5-hydroxypentyl alpha-D-glucopyranoside | C11 H22 O7 | 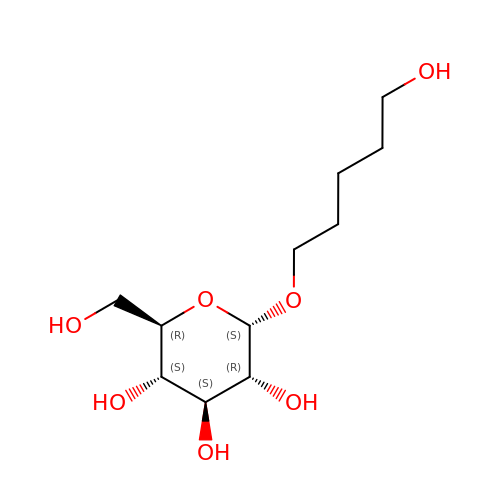TUXAGTBBQDBLQC-NZFPMDFQSA-N> MNSLYTAEGVMDKHSLWQRYVPLVRHEALRLQVRLPASVELDDLLQAGGIGLLNAVERYDALQGTAFTTYAVQRIRGAML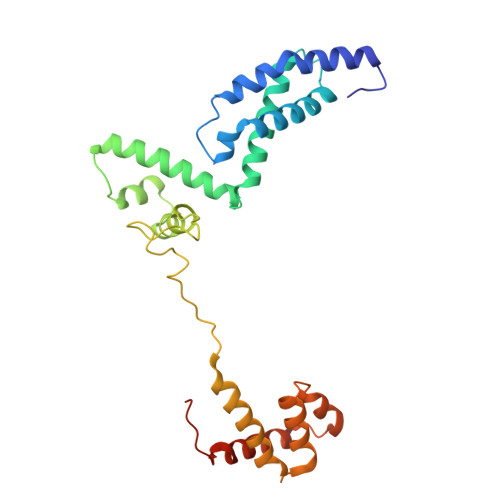DELRSRDWVPRSVRRNAREVAQAIGQLEQELGRNATETEVAERLGIDIADYRQMLLDTNNSQLFSYDEWREEHGDSIELVTDDHQRENPLQQLLDSNLRQRVMEAIETLPEREKLVLTLYYQEELNLKEIGAVLEVGESRVSQLHSQAIKRLRTKLGKLLEHHHHHH>[2x]QNSLALHKVIMVGSGGVGKS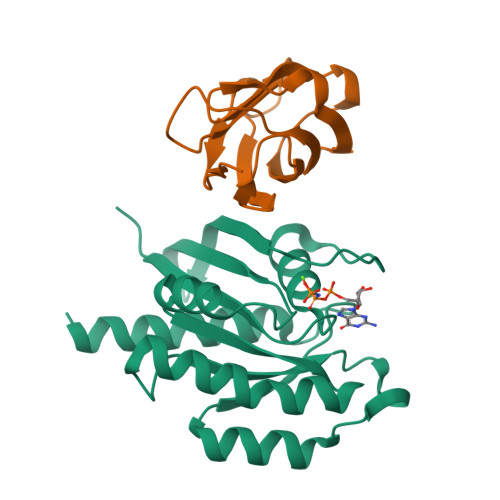ALTLQFMYDEFVEDYEPTKADSYRKKVVLDGEEVQIDILDTAGQEDYAAIRDNYFRSGEGFLCVFSITEMESFAATADFREQILRVKEDENVPFLLVGNKSDLEDKRQVSVEEAKNRAEQWNVNYVETSAKTRANVDKVFFDLMREIRARKMEDS;>[2x]MSRSRQPPLVTGISPNEGIPWTKVTIRGENLGTGPTDLIGLTICGHNCLLTAEWMSASKIVCRVGQAKNDKGDIIVTTKSGGRGTSTVSFKLLKPEKIG> SSPADSYNEGVKPWRLQPQEISPPPTANLDRSNDKVYENVTGLVKAVIEMSSKIQPAPPEEYVPMVKEVGLALRTLLATVDETIPLLPASTHREIEMAQKLLNSDLGELINKMKLAQQYVMTSLQQEYKKQMLTAAHALAVDAKNLLDVIDQARLKMLGQTR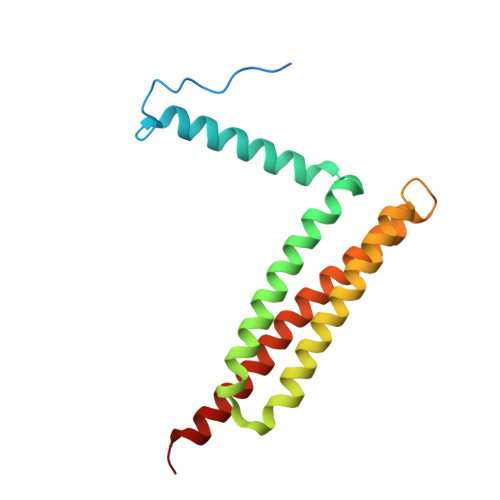PH> XDPAWYDC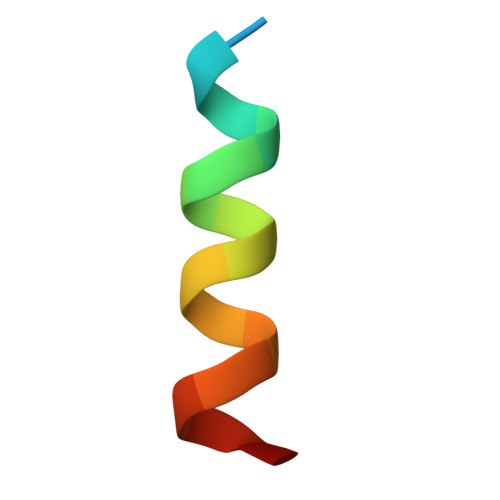ADAAWICTFX> GAGCAGCCTGTA;> TACACCGT;> CTGAT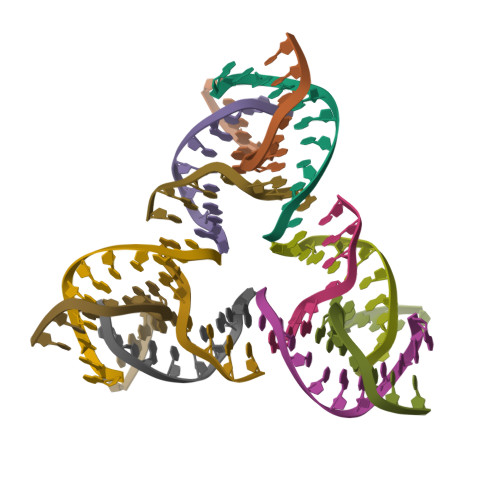GTGGCTGCT;> ACGGACATCA3-trimethylsilylpropane-1-sulfonic acid | C6 H16 O3 S Si | 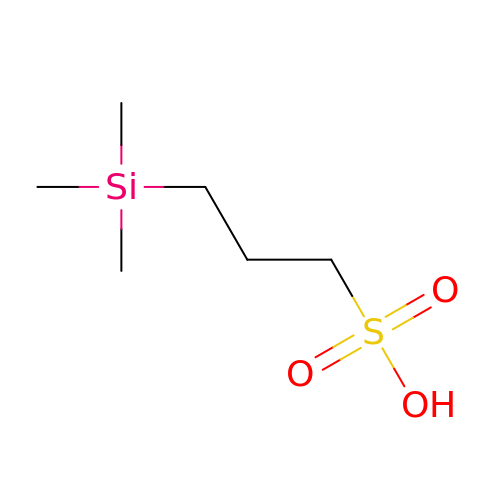TVZRAEYQIKYCPH-UHFFFAOYSA-N>[10x]MSLQGIHLSDLSYKHAILKESQYTIKRDVGTTTAVTPSSLQQEITLLCGEILYAKHADYKYAAEIGIQYISTALGSERVQQILRNSGSEVQVVLTRTYSLGKIKNNKGEDLQMLDIHGVEKSWVEEIDKEARKTMATLLKESSGNIPQ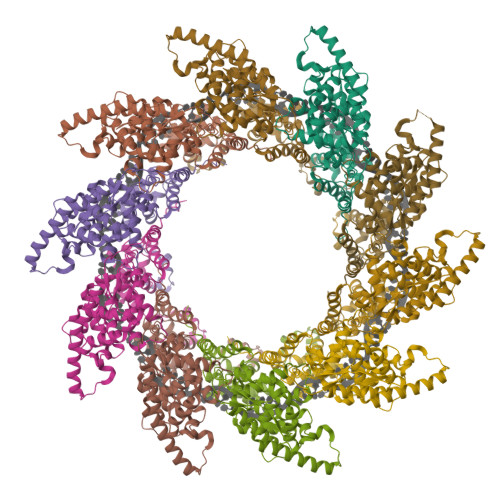NQRPSAPDTPIILLCVGALIFTKLASTIEVGLETTVRRANRVLSDALKRYPRMDIPKIARSFYDLFEQKVYHRSLFIEYGKALGSSSTGSKAESLFVNIFMQAYGAGQTMLRWGVIARSSNNIMLGHVSVQAELKQVTEVYDLVREMGPESGLLHLRQSPKAGLLSLANCPNFASVVLGNASGLGIIGMYRGRVPNTELFSAAESYAKSLKESNKINFSSLGLTDEEKEAAEHFLNVSDDSQNDYEKHHHHHH> MFGLASKGFINTSLVMVPQMNFGANLKQLKIRMKAIGSIKKITKAMKMVAASKMKAETSRLENGRNFAVGSVQKMLENESYVQKKKSTTAPKSTLLVPITSDKGLCGSVNSSIVREVKRLALNNRSAFGLLPVGEKGSSGLSRPFPDLLKSSIVNIQNVNFPTAAAIAHQVSTQGAGYDQVTLIYNHFKNAISYVVKHQELLPRAQFLNLFKYVTRHEAVEPELEYSKNYFFELYMASSV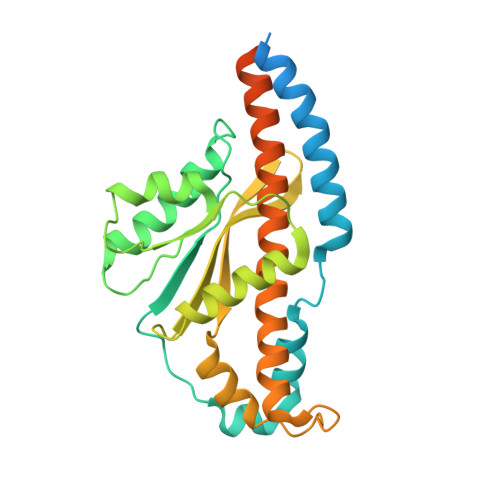YNALLNSSASEQASRMNAMENASKNAGEILSKLTLDYNKARQAKITMELIEIISGASIV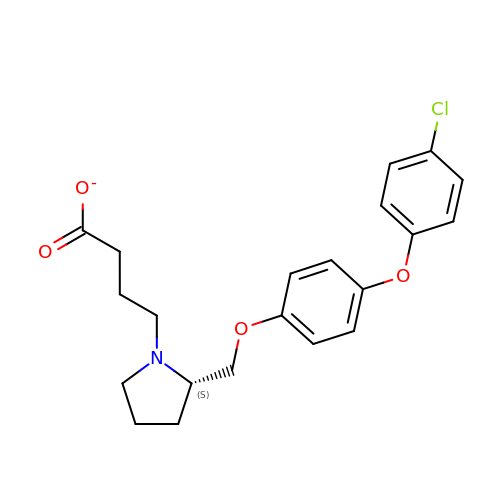4-[(2S)-2-{[4-(4-chlorophenoxy)phenoxy]methyl}pyrrolidin-1-yl]butanoate | C21 H23 Cl N O4 | PVCTYSQBVIGZRU-KRWDZBQOSA-M> GPMVHITLDPDTANPWLI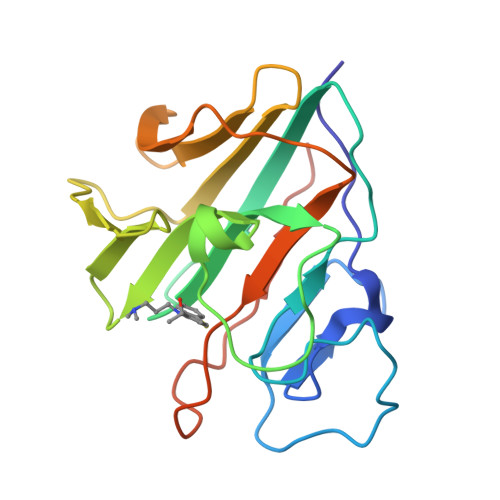LSEDRRQVRLGDTQQSIPGNEERFDSYPMVLGAQHFHSGKHYWEVDVTGKEAWALGVCRDSVRRKGHFLLSSKSGFWTIWLWNKQKYEAGTYPQTPLHLQVPPCQVGIFLDYEAGMVSFYNITDHGSLIYSFSECAFTGPLRPFFSPGFNDGGKNTAPLTLCPLNIGSQGSTDY>MQSSVNEFLTPRHIDVQVVSQTRAKITLEPLERGFGHTLGNALRRILLSSMPGCAVVEAEIDGVLHEYSAIEGVQEDVIEILLNLKGLAIKLHGRDEVTLTLAKKGSGVVTAADIQLDHDVEIINGDHVIANLADNGALNMKLKVARGRGYEPADARQSDEDESRSIGRLQLDASFSPVRRVSYVVENARVEQRTNLDKLVLDLETNGTLDPEEAIRRAATILQQQLAAFVDLKGDSEPVVEEQEDEIDPILLRPVDDLELTVRSANCLKAENIYYIGDLIQRTEVELLKTPNLGKKSLTEIKDVLASRGLSLGMRLDNWPPASLKKDDKATA[2x];> MAYSYTEKKRIRKDFSKLPDVMDVPYLLAIQLDSYREFLQAGATKEQFRDVGLHAAFKSVFPIISYSGNAALEYVGYRLGEPAFDVKECVLRGVTFAVPLRVKVRLIIFDRESSNKAIKDIKEQEVYMGEIPLMTENGTFIINGTERVIVSQLHRSPGVFFDHDRGKTHSSGKLLYSARIIPYRGSWLDFEFDPKDCVFVRIDRRRKLPASVLLRALGYSTEEILNAFYATNVFHIKGETLNLELVPQRLRGEVASIDIKDGSGKVIVEQGRRITARHINQLEKAGVSQLEVPFDYLIGRTIAKAIVHPATGEIIAECNTELTLDLLAKVAKAQVVRIETLYTNDIDCGPFISDTLKIDNTSNQLEALVEIYRMMRPGEPPTKEAAETLFGNLFFSAERYDLSAVGRMKFNRRIGRTEIEGPGVLSKEDIIDVLKTLVDIRNGKGIVDDIDHLGNRRVRCVGEMAENQFRVGLVRVERAVKERLSMAESEGLMPQDLINAKPVAAAIKEFFGSSQLSQFMDQNNPLSEITHKRRVSALGPGGLTRERAGFEVRDVHPTHYGRVCPIETPEGPNIGLINSLATYARTNKYGFLESPYRVVKDSLVTDEIVFLSAIEEADHVIAQASATLNEKGQLVDELVAVRHLNEFTVKAPEDVTLMDVSPKQVVSVAASLIPFLEHDDANRALMGSNMQRQAVPTLRADKPLVGTGMERNVARDSGVCVVARRGGVIDSVDASRVVVRVADDEVETGEAGVDIYNLTKYTRSNQNTCINQRPLVSKGDVVARGDILADGPSTDMGELALGQNMRVAFMPWNGFNFEDSICLSERVVQEDRFTTIHIQELTCVARDTKLGPEEITADIPNVGEAALNKLDEAGIVYVGAEVQAGDILVGKVTPKGETQLTPEEKLLRAIFGEKASDVKDTSLRVPTGTKGTVIDVQVFTRDGVERDSRALSIEKMQLDQIRKDLNEEFRIVEGATFERLRAALVGAKAEGGPALKKGTEITDDYLDGLERGQWFKLRMADDALNEQLEKAQAYISDRRQLLDDKFEDKKRKLQQGDDLAPGVLKIVKVYLAIKRRIQPGDKMAGRHGNKGVVSVIMPVEDMPHDANGTPVDIVLNPLGVPSRMNVGQILETHLGLAAKGLGEKINRMLEEQRKVAELRKFLHEIYNEIGGREENLDELGDNEILALAKNLRGGVPMATPVFDGAKEREIKAMLKLADLPESGQMRLFDGRTGNQFERPTTVGYMYMLKLNHLVDDKMHARSTGSYSLVTQQPLGGKAQFGGQRFGEMEVWALEAYGAAYTLQEMLTVKSDDVNGRTKMYKNIVDGDHRMEAGMPESFNVLIKEIRSLGIDIELETE;> MKDLLNLLKNQGQIEEFDAIRIGLASPEMIRSWSFGEVKKPETINYRTFKPERDGLFCAKIFGPVKDYECLCGKYKRLKHRGVICEKCGVEVALAKVRRERMGHIELASPVAHIWFLKSLPSRIGLLLDMTLRDIERVLYFESYVVIDPGMTTLEKGQLLNDEQYFEALEEFGDDFDARMGAEAVHELLNAIDLEHEIGRLREEIPQTNSETKIKKLSKRLKLMEAFQGSGNKPEWMVLTVLPVLPPDLRPLVPLDGGRFATSDLNDLYRRVINRNNRLKRLLDLAAPDIIVRNEKRMLQEAVDALLDNGRRGRAITGSNKRPLKSLADMIKGKQGRFRQNLLGKRVDYSGRSVITVGPTLRLHQCGLPKKMALELFKPFIFGKLEGRGMATTIKAAKKMVERELPEVWDVLAEVIREHPVLLNRAPTLHRLGIQAFEPVLIEGKAIQLHPLVCAAYNADFDGDQMAVHVPLTLEAQLEARALMMSTNNILSPANGEPIIVPSQDVVMGLYYMTREAINAKGEGMAFADLQEVDRAYRSGQASLHARVKVRINEKIKGEDGQLTANTRIVDTTVGRALLFQVVPAGLPFDVVNQSMKKKAISKLINHCYRVVGLKDTVIFADQLMYTGFAYSTISGVSIGVNDFVIPDEKARIINAATDEVKEIESQYASGLVTQGEKYNKVIDLWSKANDEVSKAMMANLSKEKVVDREGKEVDQESFNSMYMMADSGARGSAAQIRQLAGMRGLMAKPDGSIIETPITANFREGLNVLQYFISTHGARKGLADTALKTANSGYLTRRLVDVAQDLVVTEIDCGTEHGLLMSPHIEGGDVVEPLGERVLGRVIARDVFKPGSDEVIVPAGTLIDEKWVDFLEVMSVDEVVVRSPITCETRHGICAMCYGRDLARGHRVNIGEAVGVIAAQSIGEPGTQLTMRTFHIGGAASRTSAADNVQVKNGGTIRLHNLKHVVRADGALVAVSRSGELAVADDFGRERERYKLPYGAVISVKEGDKVDPGAIVAKWDPHTHPIVTEVDGTVAFVGMEEGITVKRQTDELTGLTNIEVMDPKDRPAAGKDIRPAVKLIDAAGKDLLLPGTDVPAQYFLPANALVNLTDGAKVSIGDVVARIPQETSKTRDITGGLPRVADLFEARRPKEPSILAEISGTISFGKETKGKRRLVITPNDGSDPYEELIPKWRHLNVFEGEQVNRGEVISDGPSNPHDILRLLGVSSLAKYIVNEIQDVYRLQGVKINDKHIETILRQMLRKVEVSESGDSSFIKGDQVELTQVLEENEQLGTEDKFPAKYERVLLGITKASLSTESFISAASFQETTRVLTEAAVTGKRDFLRGLKENVVVGRLIPAGTGLAYHSERKRQRDLGKPQRVSASEAEAALTEALNSSGN;> MARVTVEDCLDNVDNRFELVMLATKRARQLATGGKEPKVAWENDKPTVVALREIASGLVDENVVQQEDIVEDEPLFAAFDDEANTEAL;> MSGKAQQQSRLKELIARGREQGYLTYAEVNDHLPEDISDPEQVEDIIRMINDMGINVFETAPDADALLLAEADTDEAAAEEAAAALAAVESDIGRTTDPVRMYMREMGTVELLTREGEIEIAKRIEEGIREVMSAIAQFPGTVDSILADYNRIVAEGGRLSDVLSGYIDPDDGSLPAEEVEPVNLKDDSADSKEKDDEEEESDDSSDSDDEGDGGPDPEEARLRFTAVSEQLDKAKKALKKHGRGSKQATAELTGLAELFMPIKLVPKQFDALVARVRSALEGVRAQERAIMQLCVRDARMPRADFLRLFPNHETDEKWVDSVLKSKPKYAEAIERLRDDILRNQQKLAALESEVELTVAEIKEINRAMSIGEAKARRAKKEMVEANLRLVISIAKKYTNRGLQFLDLIQEGNIGLMKAVDKFEYRRGYKFSTYATWWIRQAITRSIADQARTIRIPVHMIETINKLNRISRQMLQEMGREPTPEELGERMDMPEDKIRKVLKIAKEPISMETPIGDDEDSHLGDFIEDSTMQSPIEMATSESLKESTREVLAGLTAREAKVLRMRFGIDMNTDHTLEEVGKQFDVTRERIRQIEAKALRKLRHPSRSEHLRSFLDE;> MFQSTEQALAVAYWMFEQQPGPRSSTAMVIDSLRERFDRRFIERLPSGLSPHEWQAQAVMTVRFAQRQLAAHPLELAVVRAEFARGRDFVLGLAALRDWLKPAAGPIEQRAALALLMRMFRRPPSSIREIERLSGLSKSTLHRWDKEWRERVAALLRQALLRLEEPMAQVGIVCEH

AlpA positively regulates a programmed cell death pathway linked to the virulence of Pseudomonas aeruginosa by recognizing an AlpA binding element within the promoter, then binding RNA polymerase directly and allowing it to bypass an intrinsic terminator positioned downstream. AlpA then positively regulates the cell lysis genes alpBCDE by functioning as a processive antiterminator. In particular, AlpA recognizes a putative AlpA binding element (ABE) located between the −10 and −35 elements of the alpB promoter (PalpB), binds RNAP directly, and allows it to bypass an intrinsic termination site (tB) positioned downstream of PalpB. Like 21Q, AlpA forms a narrow ring inside the RNA exit channel and renders RNAP resistant to termination signals by prohibiting RNA hairpin formation.

To obtain the structure of an AlpA-loading complex, we used a nucleic-acid scaffold corresponding to positions −31 to + 31 of promoter PalpB. The scaffold contains an ABE, a consensus −10-like sequence, a 13-bp transcription bubble maintained in the unwound state by having non-complementary sequences on nontemplate and template strands, and a 12-nt RNA. 3D classification revealed the structure of the AlpA-loading complex, determined at a nominal resolution of 3.3 Å. Unlike 21Q, only one AlpA molecule binds to the ABE and RNA exit channel in the loading complex. In addition, σR2 binds to the −10-like sequence in the same way as in 21Q-loading complex and RNAP-promoter open complex, in accordance with the observation that the −10-like sequence is critical for AlpA-dependent transcription antitermination. σ70 conserved regions σR3, σR3.2 and σR4 are displaced from RNAP, probably due to the steric clashes between σR3.2, σR4, and the 5′ end of nascent RNA, consistent with the fact that σR3, σR3.2 and σR4 are dispensable for σ-dependent pause. The N-terminal segment of AlpA, including L1, L2 and H2 forms a ring-like structure, while the C-terminal segment of AlpA, including H7 and H8, forms a helix-turn-helix motif. In the AlpA-loading complex structure, the helix-turn-helix motif formed by H7 and H8 participates in the recognition of ABE. Specifically, residues R128, K138, S139, T140 and H142 are positioned in the major groove, potentially making interactions with DNA that could enable sequence readout. Our structure of the AlpA-loading complex reveals that the N-terminal segment of AlpA forms a ring-like structure and contacts various elements of the RNA exit channel. In particular, H3 sits on the exterior opening of the RNA exit channel and interacts with the dock, while H2 inserts into the RNA exit channel and interacts with the zipper, lid, and zinc binding domain (ZBD).>GSRNQSPPQMMAQQGMHMQWTDQSFIEMMTPHHQDAIDMAEMALQKAEHPELKKLARNIIRD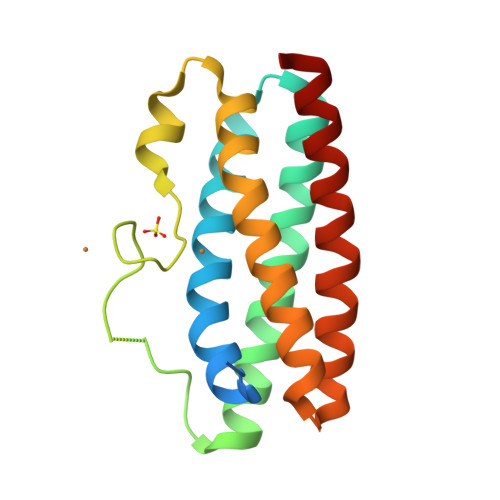QEREIKEMKTWYQQWFKRPVPALSSQGMMGMHQGHGMMAMDLDALATAQNFDREFIRQMIPHHQMAVMMASNLKTNTERPEMDKLMDDIIRSQSAEIKQMKQWYQNWYGQ[2x]>GSSHHHHHHSSGLVPRGSMAEKFESRGIEEASSEVPTQRRCGAMEVHHRLLRSASYVRERDQIENLALKYKQGFRAISRMEIVKIPVVVHVVWNEEEENISDAQIQSQIDILNKDFRKLNSDVSQVPSVWSNLIADLGIEFFLATKDPNGNQTTGITRTQTSVTFFTTSDEVKFASSGGEDAWPADRYLNIWVCHVLKSEIGQDILGYAQFPGGPAETDGVVIVDAAFGTTGTALPPFDKGRTATHAIGHWLNLYHIWGD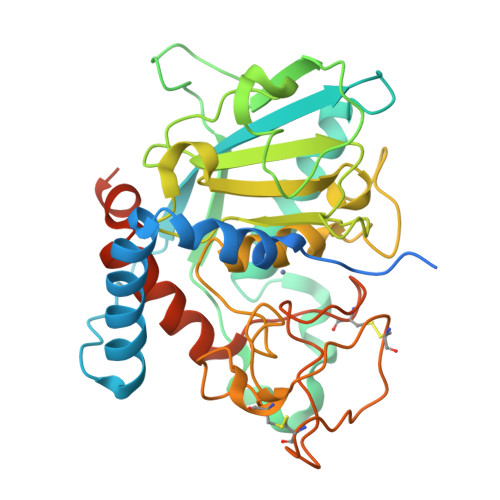ELRFEDPCSRSDEVDDTPNQADPNFGCPSYPHVSCSNGPNGDMFMNYMDYVDDKCMVMFTQGQATRVNACLDGPRSSFLARVEETEKKEAPSKREMPMPR[14x]> ACGGACAGCAC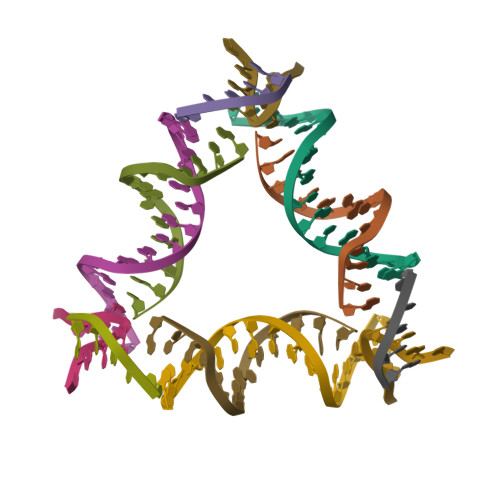GTGTA;> CACACCGT;> GTGCACGTGCTGT;> CTGTG>GGSMSNPDYCIPNFSQTVNERTIIDIFTICRYRSPLVVFCLSHNELAKKYAQDVSMSSGTHVHIIDGSVEITVSLYRTFRTIATQLLGRMQIVVFVTVDKSVVSTQVMKSIAWAFRGSFVELRNQSVDSSTLVSKLENLVSFAPLYNVPKCGPDYYGPTVYSELLSLATNARTHWYATIDYSMFTRSVLTGFVAKYFNEEAVPIDKRIVSIVGYNPPYVWTCLRHGIRPTYIEKSLPNPGGKGPFGLILPVINELVLKSKVKYVMHNPQIKLLCLDTFMLSTSMNILYIGAYPATHLLSLQLNGWTILAFDPKITSDWTDAMAKATGAKVIGVSKEFDFKSFSVQANQLNMFQNSKLSVIDDTWVETDYEKFQSEKQAYFEWLIDRTSIDVRLISMKWNRSKDTSVSHLLALLPQPYGASIREMRAFFHKKGASDIKILAAETEKYMDDFTAMSVSDQINTQKFMHCMITTVGDALKMDLDGGRAVIASYSLSNSSNSKERVLKFLSDANKAKA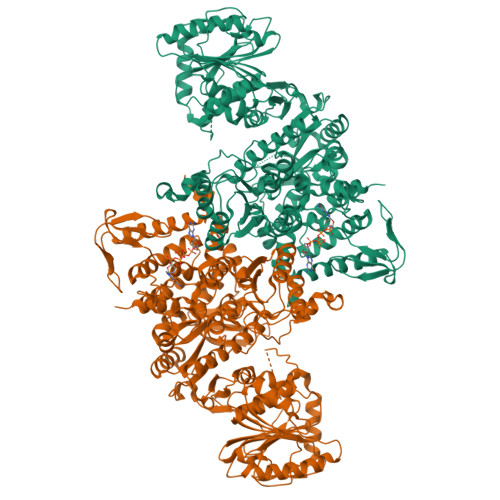MVVFGAPNTHRLAYAKKVGLVLDSAIKMSKDLITFSNPTGRRWRDYGYSQSELYDAGYVEITIDQMVAYSSDVYNGVGYFANSTYNDLFSWYIPKWYVHKRMLMQDIRLSPAALVKCFTTLIRNICYVPHETYYRFRGILVDKYLRSKNVDPSQYSIVGSGSKTFTVLSHFEVPHECGPLVFEASTDVNISGHLLSLAIAAHFVASPMILWAEQMKYMAVDRMLPPNLDKSLFFDNKVTPSGALQRWHSREEVLLAAEICESYAAMMLNNKHSPDIIGTLKSAINLVFKI[4x]The sulfonamides (sulfas) are the oldest class of antibacterial drugs and inhibit the bacterial dihydropteroate synthase (DHPS, encoded by folP), through chemical mimicry of its co-substrate p-aminobenzoic acid (pABA). Resistance to sulfa drugs is mediated either by mutations in folP or acquisition of sul genes, which code for sulfa-insensitive, divergent DHPS enzymes. DHPS catalyzes the condensation of para-aminobenzoic acid (pABA) and 6-hydroxymethyl-7,8-dihydropterin pyrophosphate (DHPP), producing 7,8-dihydropteroic acid (7,8-DHP); this compound is further transformed, ultimately leading to tetrahydrofolate, an essential precursor for DNA and RNA synthesis. All three Sul enzymes adopted the (ɑ/β)8 TIM barrel fold also shared by DHPS.

The Sul2·7,8-DHP·Mg2+·PPi complex structure provided essential insights into the molecular architecture of the Sul enzyme’s fully ligand-occupied active state, containing both products of the enzymatic reaction and with loops 1, 2 and 3 engaged in ligand interactions. In comparison to the Sul1 structure, the pABA molecule formed fewer interactions with the Sul2 enzyme and occupied the more solvent-exposed positively charged region of the active site pocket. In this conformation, the pABA carboxylate forms interactions with Ser214, the p-amino group with Ser52, and with aliphatic region of Lys213 and the sidechain of Phe179. All the protein-ligand interactions observed in the Sul2·7,8-DHP·Mg2+·PPi complex were consistent with those observed in the Sul3·DHP+·pABA·Mg2+·PPi complex, including the hydrophobic interaction between pABA and Phe177. The pterin group and the pABA group of the ligands bound to Sul2/Sul3 or DHPS occupied the same spatial locations in all analyzed structures. Leveraging our structure of the Sul2·7,8-DHP·Mg2+·PPi complex, we modeled 12 clinically relevant sulfonamides in the Sul2 active site through superposition with the pABA region of 7,8-DHP. This analysis showed that all 12 compounds would pose a steric clash with the Phe residue of ɑ6 helix, including the most primitive sulfa sulfanilamide, whose structure is the closest mimic to pABA. The modeling suggested that the sulfonamide nitrogen would be positioned 2.1 Å distance from the Phe residue, resulting in an unfavorable clash. The modeling further suggested that the N-acyl substituents off the sulfonamide nitrogen that define the different compounds would exacerbate the clash with F179, at least using their energy-minimized conformations in our models.

>[2x]MNKSLIIFGIVNITSDSFSDGGRYLAPDAAIAQARKLMAEGADVIDLGPASSNPDAAPVSSDTEIARIAPVLDALKADGIPVSLDSYQPATQAYALSRGVAYLNDIRGFPDAAFYPQLAKSSAKLVVMHSVQDGQADRREAPAGDIMDHIAAFFDARIAALTGAGIKRNRLVLDPGMGFFLGAAPETSLSVLARFDELRLRFDLPVLLSVSRKSFLRALTGRGPGDVGAATLAAELAAAAGGADFIRTHEPRPLRDGLAVLAALKETARIR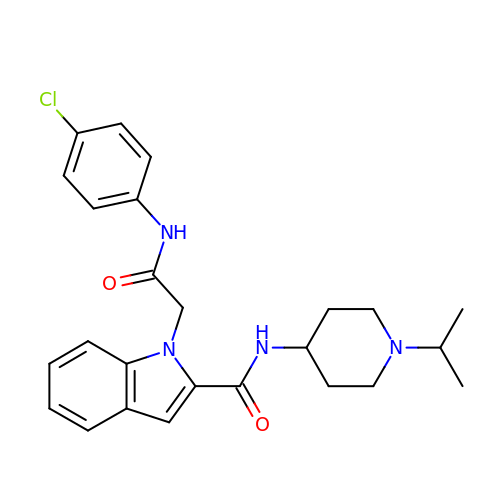1-{2-[(4-CHLOROPHENYL)AMINO]-2-OXOETHYL}-N-(1-ISOPROPYLPIPERIDIN-4-YL)-1H-INDOLE-2-CARBOXAMIDE | C25 H29 Cl N4 O2 | BDLMBQRBNPDCSS-UHFFFAOYSA-N> MVAITVQGAQLIKRVVERFYPGIAFNINEGACYIYKFSDHIRRIRMKHGTKYRRQAEEIIRNISLRKERLYGIPVLDEVEWKYVFDGQTFQSYAFEVYVNSILPWSELDPEEEFLRNYRVSREMTEVEKFIEFRAKNEMQIYGDIPIKVWCCFINELSAELKHVPLGMQVMADFVNRFDSPFHQGNRDLSNLEDFQVAYTTPLLFEMCCMESILEFNIKMRMREEEISALEFGDMKVDPVGLLREFFILCLPHPKKINNVLRAPYSWFVKMWGVGADPIVVLQSTAGDDRNSKDVFYDKFRTEPNRYKALFRSSFYNESRRMNEEKILEAVKYSQKLGSHDRRLPLFEKMLKTVYTTPFYPHKSSNMILASFLLSIQTITGYGRAWVKNVSTEFDKQLKPNPSNLVQDVSDLTREFFKQAYVEAKERREEIVKPEDLYTSMLRLARNTSSGFSTEIYVKKRFGPRLRDKDLIKINSRIKALVIFTKGHTVFTDEELHKKYNSVELYQTKGSRDVPIKATRTIYSINLSVLVPQLIVTLPLNEYFSRVGGITSPDYKKIGGKVIVGDLEATGSRVMDAADCFRNSADRDIFTIAIDYSEYDTHLTRHNFRTGMLQGIREAMAPYRDLRYEGYTLEQIIDFGYGEGRVANTLWNGKRRLFKTTFDAYIRLDESERDKGSFKVPKGVLPVSSVDVANRIAVDKGFDTLIAATDGSDLALIDTHLSGENSTLIANSMHNMAIGTLMQREVGREQPGVLTFLSEQYVGDDTLFYTKLHTTDTKVFDKVAASIFDTVAKCGHEASPSKTMMTPYSVEKTQTHAKQGCYVPQDRMMIISSERRKDIEDVQGYVRSQVQTMITKVSRGFCHDLAQLILMLKTTFIGAWKMKRTIKEDAMYRDRKFDSNDEDGFTLIQIRNPLALYVPIGWNGYGAHPAALNIVMTEEMYVDSIMISKLDEIMAPIRRIVHDIPPCWNETQGDKRGLISATKMSFFSKMARPAVQAALSDPQIINLVEELPLGEFSPGRISRTMMHSALLKESSARTLLSSGYELEYQKALNSWITQVSMRLGEESGVISTSYAKLFDVYFEGELDGAPHMFPDQNLSPQFYIQKMMIGPRVSSRVRNSYVDRIDVILRKDVVMRGFITANTILNVIEKLGTNHSVGDLVTVFTLMNIETRVAEELAEYMTSEKIRFDALKLLKKGIAGDEFTMSLNVATQDFIDTYLAYPYQLTKTEVDAISLYCTQMIMLRAALGLPKKKMKIVVTDDAKKRYKIRLQRFRTHVPKIKVLKKLIDPNRMTVRNLENQFV;>[10x]MAAQNEQRPERIKTTP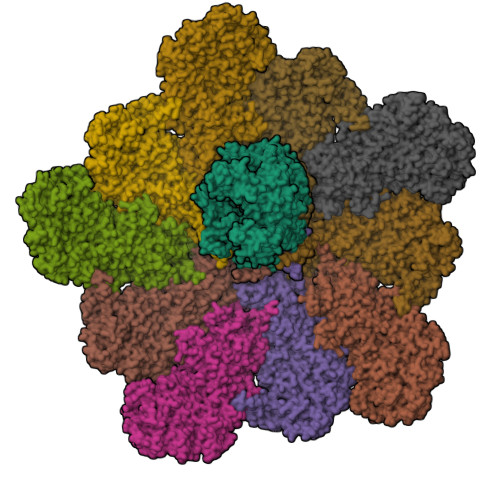YLEGDVLSSDSGPLLSVFALQEIMQKVRQVQADYMTATREVDFTVPDVQKILDDIKALAAEQVYKIVKVPSISFRHIVMQSRDRVLRVDTYYEEMSQVGDVITEDEPEKFYSTIIKKVRFIRGKGSFILHDIPTRDHRGMEVAEPEVLGVEFKNVLPVLTAEHRAMIQNALDGSIIENGNVATRDVDVFIGACSEPVYRIYNRLQGYIEAVQLQELRNSIGWLERLGHRKRITYSQEVLTDFRRQDTIWVLALQLPVNPQVVWDVPRSSIANLIMNIATCLPTGEYIAPNPRISSITLTQRITTTGPFAILTGSTPTAQQLNDVRKIYLALMFPGQIILDLKIDPGERMDPAVRMVAGVVGHLLFTAGGRFTNLTQNMARQLDIALNDYLLYMYNTRVQVNYGPTGEPLDFQIGRNQYDCNVFRADFATGTGYNGWATIDVEYREPAPYVHAQRYIRYCGIDSRELINPTTYGIGMTYHCYNEMLRMLVAAGKDSEAAYFRSMLPFHMVRFARINQIINEDLHSVFSLPDDMFNALLPDLIAGAHQNADPVVLDVSWISLWFAFNRSFEPTHRNEMLEVAPLIESVYASELSVMKVDMRHLSLMQRRFPDVLIQARPSHFWKAVLNDSPEAVKAVMNLSHSHNFINIRDMMRWVMLPSLQPSLKLALEEEAWAAANDFEDLMLTDQVYMHRDMLPEPRLDDIERFRQEGFYYTNMLEAPPEIDRVVQYTYEIARLQANMGQFRAALRRIMDDDDWVRFGGVLRTVRVKFYDARPPDDVLQGLPFSYDTNERGGLAYATIKYATETTIFYLIYNVEFSNTPDSLVLINPTYTMTKVFINKRIVERVRVGQILAVLNRRFVAYKGKMRIMDITQSLKMGTKLAAPTV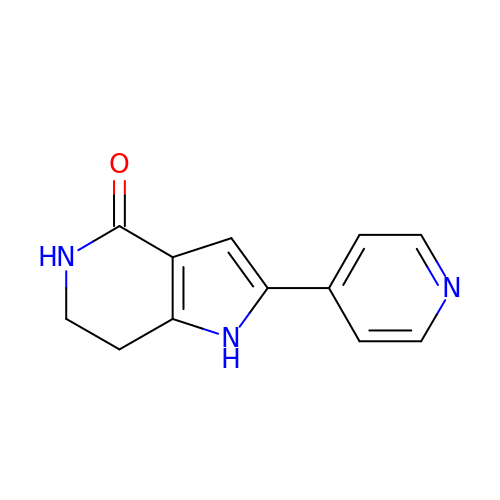2-(pyridin-4-yl)-1,5,6,7-tetrahydro-4H-pyrrolo[3,2-c]pyridin-4-one | C12 H11 N3 O | DKXHSOUZPMHNIZ-UHFFFAOYSA-N>[4x]MCLPTIRKIAIIGAGPSGLVTAKALLAEKAFDQVTLFERRGSPGGVWNYTSTLSNKLPVPSTNPILTTEPIVGPAALPVYPSPLYRDL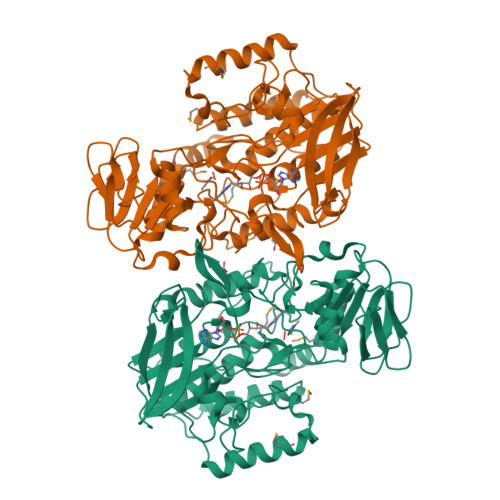QTNTPIELMGYCDQSFKPQTLQFPHRHTIQEYQRIYAQPLLPFIKLATDVLDIEKKDGSWVVTYKGTKAGSPISKDIFDAVSICNGHYEVPYIPNIKGLDEYAKAVPGSVLHSSLFREPELFVGESVLVVGGASSANDLVRHLTPVAKHPIYQSLLGGGDIQNESLQQVPEITKFDPTTREIYLKGGKVLSNIDRVIYCTGYLYSVPFPSLAKLKSPETKLIDDGSHVHNVYQHIFYIPDPTLAFVGLALHVVPFPTSQAQAAFLARVWSGRLKLPSKEEQLKWQDELMFSLSGANNMYHSLDYPKDATYINKLHDWCKQATPVLEEEFPSPYWGEKERSIRENMWSIRAKFFGIEPPK(R)-3-(Benzylthio)-2-(3-(4-chloro-[1,1':2',1'':3'',1'''-quaterphenyl]-4'''-carbonyl)-3-(4-methylbenzyl)ureido)propanoic 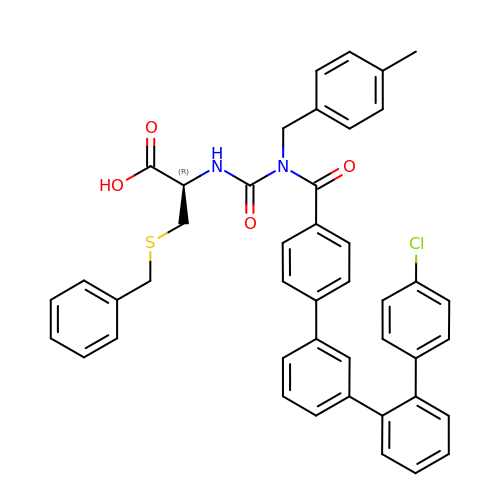acid | C44 H37 Cl N2 O4 S | COHZWEMEHOCPAK-RWYGWLOXSA-N> XTTWEAWDXAIAE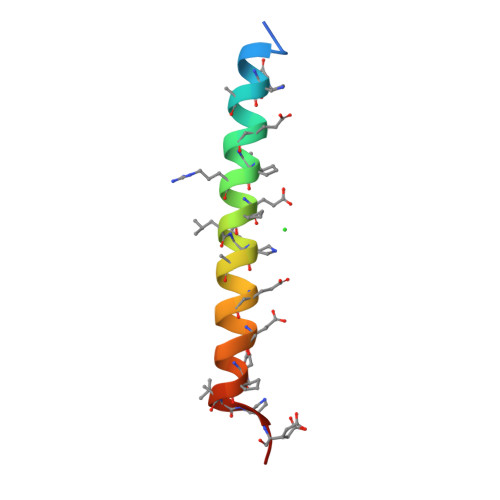YAXRIEXLIXAAQEQQEKNEXALXELX> GGLEKDFLPLYFGWFLTKKSSETLRKAGQVFLEELGNHKAFKKELRHFISGDEPKEKLELVSYFGKRPPGVLQCTTKFCDYG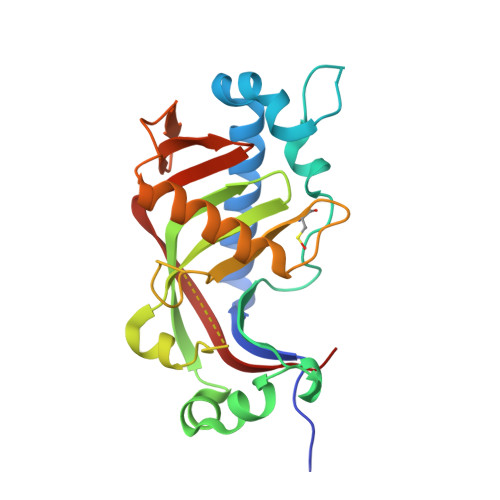KAAGAEEYAQQEVVKRSYGKAFKLSISALFVTPKTAGAQVVLTDQELQLWPSDLDKPSASEGLPPGSRAQVTLGCAADVQPVQTGLDLLDILQQVKGGSQGEAVGELPRGKLYSLGKGRWMLSLTKKMEVKAIFTGYYG> GLGDLIEGVVEGVTRNALTPLTPANNLPDTQSSGPAHSKETPALTAVETGATNPLV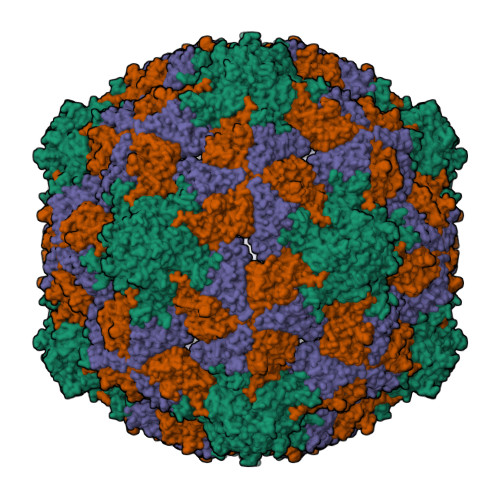PSDTVQTRHVIQKRTRSESTVESFFARGACVAIIEVDNDAPTKRASKLFSVWKITYKDTVQLRRKLEFFTYSRFDMEFTFVVTSNYTDANNGHALNQVYQIMYIPPGAPIPGKWNDYTWQTSSNPSVFYTYGAPPARISVPYVGIANAYSHFYDGFAKVPLAGQASTEGDSLYGAASLNDFGSLAVRVVNDHNPTKLTSKIRVYMKPKHVRVWCPRPPRAVPYYGPGVDYKDGLAPLPEKGLTTY;> SPNIEACGYSDRVMQLTLGNSTITTQEAANSVVAYGRWPEYIKDSEANPVDQPTEPDVAACRFYTLDTVTWRKESRGWWWKLPDALKDMGLFGQNMFYHYLGRAGYTVHVQCNASKFHQGALGVFAVPEMCLAGDSTTHMFTKYENANPGEKGGEFKGSFTLDTNATNPARNFCPVDYLFGSGVLAGNAFVYPHQIINLRTNNCATLVLPYVNSLSIDSMTKHNNWGIAILPLAPLDFATESSTEIPITLTIAPMCCEFNGLRNITVPRTQ;> GLPVLNTPGSNQYLTADNYQSPCAIPEFDVTPPIDIPGEVRNMMELAEIDTMIPLNLTNQRKNTMDMYRVELNDAAHSDTPILCLSLSPASDPRLAHTMLGEILNYYTHWAGSLKFTFLFCGSMMATGKLLVSYAPPGAEAPKSRKEAMLGTHVIWDIGLQSSCTMVVPWISNTTYRQTINDSFTEGGYISMFYQTRVVVPLSTPRKMDILGFVSACNDFSVRLLRDTTHISQEAMPQ>[2x]GIDPFTGIDPFTGTQACITAASAVSGIIADLDTTIMFATAGTLNREGAETFADHREG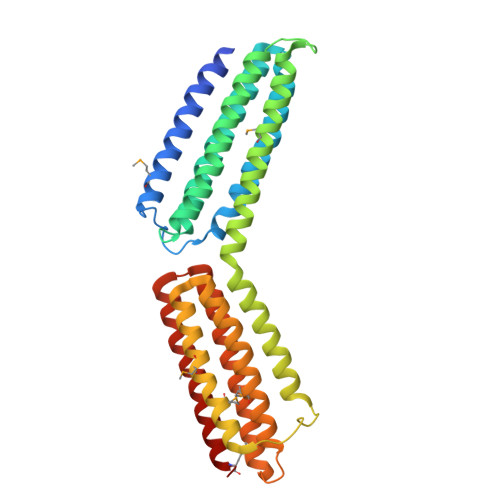ILKTAKVLVEDTKVLVQNAAGSQEKLAQAAQSSVATITRLADVVKLGAASLGAEDPETQVVLINAVKDVAKALGDLISATKAAAGKVGDDPAVWQLKNSAKVMVTNVTSLLKTVKAVEDEATKGTRALEATTEHIRQELAVFCSPEPPAKTSTPEDFIRMTKGITMATAKAVAAGNSCRQEDVIATANLSRRAIADMLRACKEAAFHPEVAPDVRLRALHYGRECANGYLELLDHVLLTLQKPNPDLKQQLTGHSKRVAGSVTELIQAAEAMKGT> ENLKLGFLVKQPEEPWFQTEWKFADKAGKDLGFEVIKIAVPDGEKTLNAIDSLAASGAKGFVICTPDPKLGSAIVAKARGYDMKVIAVDDQFVNAKGKPMDTVPLVMMAATKIGERQGQELYKEMQKRGWDVKESAVMAITANELDTARRRTTGSMDALKAAGFPEKQIYQVPTKSNDIPGAFDAANSMLVQHPEVKHWLIVGMNDSTVLGGVRATEGQG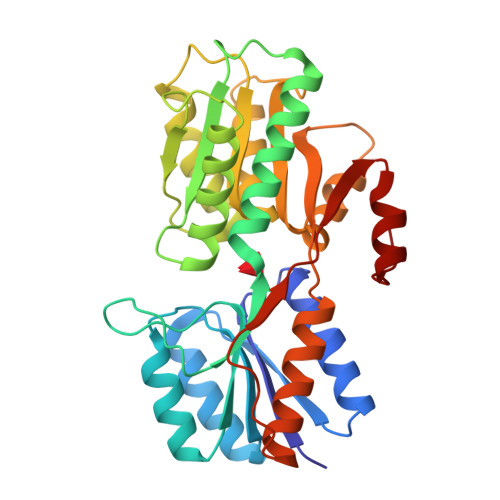FKAADIIGIGINGVDAVSELSKAQATGFYGSLLGSPDVHGYKSSEMLYNWVAKDVEPPKFTEVTDVVLITRDNFKEELEKKGLGGK>GEADM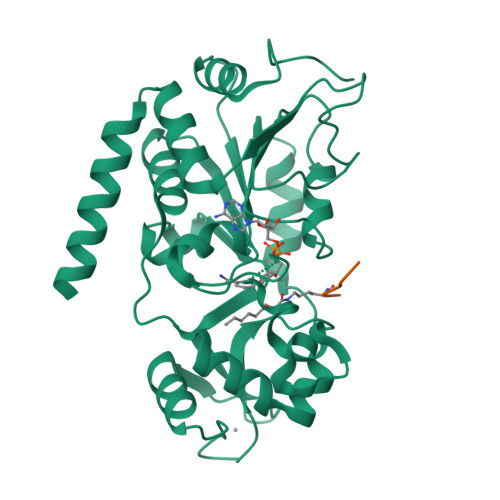DFLRNLFSQTLSLGSQKERLLDELTLEGVARYMQSERCRRVICLVGAGISTSAGIPDFRSPSTGLYDNLEKYHLPYPEAIFEISYFKKHPEPFFALAKELYPGQFKPTICHYFMRLLKDKGLLLRCYTQNIDTLERIAGLEQEDLVEAHGTFYTSHCVSASCRHEYPLSWMKEKIFSEVTPKCEDCQSLVKPDIVFFGESLPARFFSCMQSDFLKVDLLLVMGTSLQVQPFASLISKAPLSTPRLLINKEKAGQSDPFLGMIMGLGGGMDFDSKKAYRDVAWLGECDQGCLALAELLGWKKELEDLVRREHASIDAQS[2x];>[2x]RAAKT>[4x]MEIAFLLNGETRRVRIEDPTQSLLEWLRAEGLTGTKEGCNEGDCGACTVMIRDAAGSRAVNACLMMLPQIAGKALRTIEGIAAPDGRLHPVQQAMIDHHGSQCGFCTPGFIVSMAAAHDRDRKDYDDLLAGNLCRCTGYAPILRAAEAAAGEPPADWLQADAAFTLAQLSSGVRGQTAPAFLPETSDALADWYLAHPEATLIAGGTDVSLWVTKALRDLPEVAFLSHCKDLAQIRETPDGYGIGAGVTIAALRAFAEGPHPALAGLLRRFASEQVRQVATIGGNIANGSPIGDGPPALIAMGASLTLRRGQERRRMPLEDFFLEYRKQDRRPGEFVESVTLPKSAPGLRCYKLSKRFDQDISAVCGCLNLTLKGSKIETARIAFGGMAGVPKRAAAFEAALIGQDFREDTIAAALPLLAQDFTPLSDMRASAAYRMNAAQAMALRYVRELSGEAVAVLEVMP;>MSVGKPLPHDSARAHVTGQARYLDDLPCPANTLHLAFGLSTEASAAITGLDLEPVRESPGVIAVFTAADLPHDNDASPAPSPEPVLATGEVHFVGQPIFLVAATSHRAARIAARKARITYAPRPAILTLDQALAADSRFEGGPVIWARGDVETALAGAAHLAEGCFEIGGQEHFYLEGQAALALPAEGGVVIHCSSQHPSEIQHKVAHALGLAFHDVRVEMRRMGGGFGGKESQGNHLAIACAVAARATGRPCKMRYDRDDDMVITGKRHDFRIRYRIGADASGKLLGADFVHLARCGWSADLSLPVCDRAMLHADGSYFVPALRIESHRLRTNTQSNTAFRGFGGPQGALGMERAIEHLARGMGRDPAELRALNFYDPPERGGLSAPPSPPEPIATKKTQTTHYG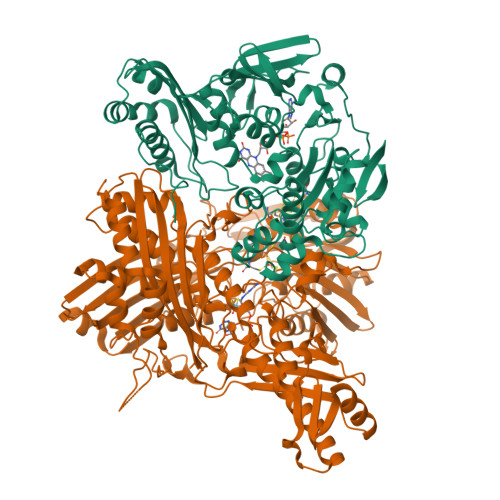QEVADCVLGELVTRLQKSANFTTRRAEIAAWNSTNRTLARGIALSPVKFGISFTLTHLNQAGALVQIYTDGSVALNHGGTEMGQGLHAKMVQVAAAVLGIDPVQVRITATDTSKVPNTSATAASSGADMNGMAVKDACETLRGRLAGFVAAREGCAARDVIFDAGQVQASGKSWRFAEIVAAAYMARISLSATGFYATPKLSWDRLRGQGRPFLYFAYGAAITEVVIDRLTGENRILRTDILHDAGASLNPALDIGQIEGAYVQGAGWLTTEELVWDHCGRLMTHAPSTYKIPAFSDRPRIFNVALWDQPNREETIFRSKAVGEPPFLLGISAFLALHDACAACGPHWPDLQAPATPEAVLAAVRRAEGRA[4x]>[2x]MRKLCSLDNGDCDQFCHEEQNSVVCSCARGYTLADNGKACIPTGPYPCGKQTLERRKR;>[2x]IVG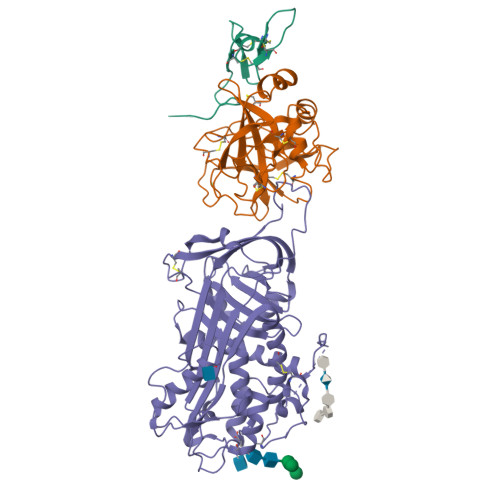GQECKDGECPWQALLINEENEGFCGGTILSEFYILTAAHCLYQAKRFKVRVGDRNTEQEEGGEAVHEVEVVIKHNRFTKETYDFDIAVLRLKTPITFRMNVAPACLPERDWAESTLMTQKTGIVSGFGRTHEKGRQSTRLKMLEVPYVDRNSCKLSSSFIITQNMFCAGYDTKQEDACQGDAGGPHVTRFKDTYFVTGIVSWGEGCARKGKYGIYTKVTAFLKWIDRSMKTRGLPKAK;>[2x]LLIGFWDCVTCHGSPVDICTAKPRDIPMNPMCIYRSPEKKATEDEGSEQKIPEATNRRVWELSKANSRFATTFYQHLADSKNDNDNIFLSPLSISTAFAMTKLGACNDTLQQLMEVFKFDTISEKTSDQIHFFFAKLNCRLYRKANKASKLVSANRLFGDKSLTFNETYQDISELVYGAKLQPLDFKENAEQSRAAINKWVSNKTEGRITDVIPSEAINELTVLVLVNTIYFKGLWKSKFSPENTRKELFYKADGESCSASMMYQEGKFRYRRVAEGTQVLELPFKGDDITMVLILPKPEKSLAKVEKELTPEVLQEWLDELEEMMLVVHMPRFRIEDGFSLKEQLQDMGLVDLFSPAASALPGIVAEGRDDLYVSDAFHKAFLEVNEEGSEAAASTAVVIAGRSLNPNRVTFKANRPFLVFIREVPLNTIIFMGRVANPCVK> MRGSHHHHHHGSGDLVAWNKKDDRRTLWTTPDTSPNCKMSTEKDSKLTLTLTKCGSQVLGNVSLLAVTGEYHQMTATTKKDVKISLLFDENGILLPSSSLSKDYWNYRSDDSIVSQKYNNAVPFMPNLTAYPKPSAQNAKNYSRTKIISNVYLGALTYQPVIITIAFNQETENGCAYSITFTFTWQKDYSA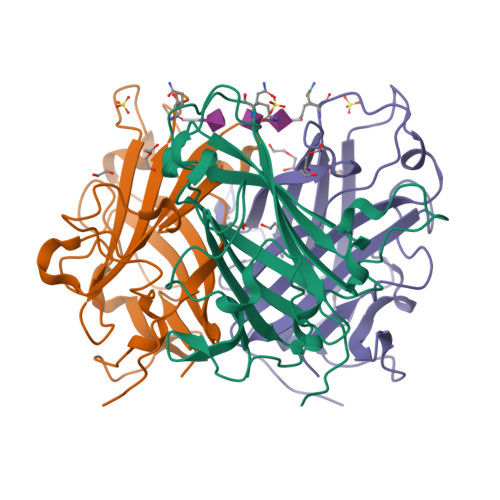QQFDVTSFTFSYLTQENKDKD> MSHNLFTEEDNNKTIRMVIGETFTIELESNPTTGYTWLRSGLAGTELSDCTFAIQSKFNNRAPHDNHKNHRR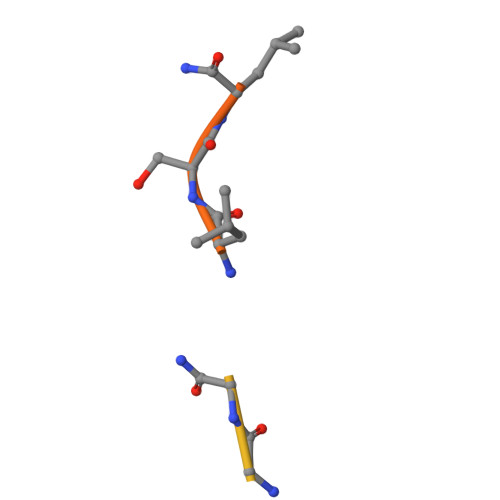LLVGAGGTMVLEVKALKAGKHTLSLAYGRPWVGFNAAAKRYNIHVEATA>MQQKSDNVVSHYVFEAPVRIWHWLTVLCMAVLMVTGYFIGKPLPSVSGEATYLFYMGYIRLIHFSAGMVFTVVLLMRIYWAFVGNRYSRELFIVPVWRKSWWQGVWYEIRWYLFLAKRPSADIGHNPIAQAAMFGYFLMSVFMIITGFALYSEHSQYAIFAPFRYVVEFFYWTGGNSMDIHSWHRLGMWLIGAFVIGHVYMALREDIMSDDTVISTMVNGYRSHKFGKISNKERS[2x];>[4x]MSTQYETQGYTINNAGRRLVVDPITRIEGHMRCEVNINDQNVITNAVSCGTMFRGLEIILQGRDPRDAWAFVERICGVCTGVHALASVYAIEDAIGIKVPDNANIIRNIMLATLWCHDHLVHFYQLAGMDWIDVLDALKADPRKTSELAQSLSSWPKSSPGYFFDVQNRLKKFVEGGQLGIFRNGYWGHPQYKLPPEANLMGFAHYLEALDFQREIVKIHAVFGGKNPHPNWIVGGMPCAINIDESGAVGAVNMERLNLVQSIITRTADFINNVMIPDALAIGQFNKPWSEIGTGLSDKCVLSYGAFPDIANDFGEKSLLMPGGAVINGDFNNVLPVDLVDPQQVQEFVDHAWYRYPNDQVGRHPFDGITDPWYNPGDVKGSDTNIQQLNEQERYSWIKAPRWRGNAMEVGPLARTLIAYHKGDAATVESVDRMMSALNLPLSGIQSTLGRILCRAHEAQWAAGKLQYFFDKLMTNLKNGNLATASTEKWEPATWPTECRGVGFTEAPRGALGHWAAIRDGKIDLYQCVVPTTWN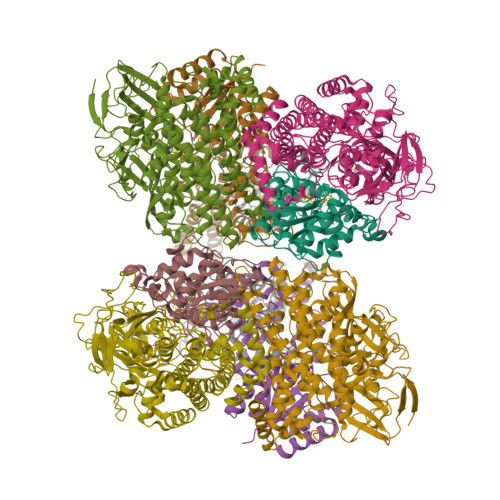ASPRDPKGQIGAYEAALMNTKMAIPEQPLEILRTLHSFDPCLACSTH;>[4x]LENKPRIPVVWIHGLECTGCTESFIRSAHPLAKDVILSLISLDYDDTLMAAAGTQAEEVFEDIITQYNGKYILAVEGNPPLGEQGMFCISSGRPFIEKLKRAAAGASAIIAWGTCASWGCVQAARPNPTQATPIDKVITDKPIIKVPGCPPIPDVMSAIITYMVTFDRLPDVDRMGRPLMFYGQRIHDKCYRRAHFDAGEFVQSWDDDAARKGYCLYKMGCKGPTTYNACSSTRWNDGVSFPIQSGHGCLGCAENGFWDRGSFYSRVVDIPQMGTHSTADTVGLTALGVVAAAVGVHAVASAVDQRRRHNQQPTETEHQPGNEDKQARSHHHHHH> MASYLKLKAQEETWLQRHSRLILAILAGLGSLLTAYLTYTKLTEQPAAFCTGDGGSDLVLSSRWAEFLGIPTAAVGLLGFLGVLALAVLPDGLPLVKRWRWPALFGLVSAMTAFEMYMLYLMVAVLRQFCMYCTTAIILVAGLGLVTVL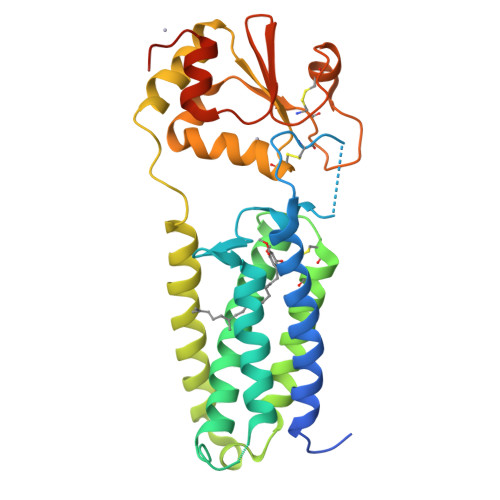GHRWLDGGKLAFSYILVAFLTLVTTIGVYANQVPPPSPLAVGLAAHLRQIGGTMYGAYWCPHCQDQKELFGAAFDQVPYVECSPNGPGTPQAQECTEAGITSYPTWIINGRTYTGVRSLEALAVASGYPLEEGRLEHHHHHH> MEGNHEEPQGGLEELSGRWHSVALASNKSDLIKPWGHFRVFIHSMSAKDGNLHGDILIPQDGQCEKVSLTAFKTATSNKFDLEYWGHNDLYLAEVDPKSYLILYMINQYNDDTSLVAHLMVRDLS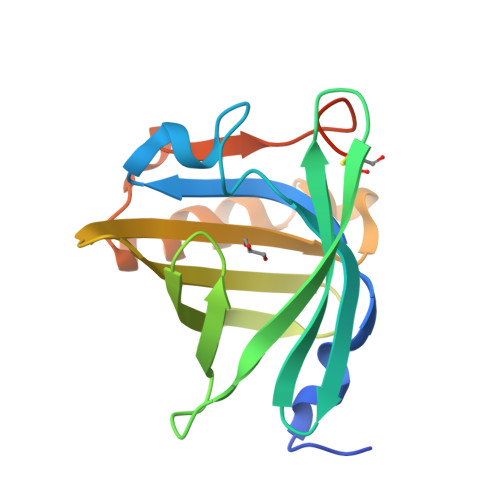RQQDFLPAFESVCEDIGLHKDQIVVLSDDDRCQGSRDLEHHHHHH>MKELNDLEKKYNAHIGVYALDTKSGKEVKFNSDKRFAYASTSKAINSAILLEQVPYNKLNKKVHINKDDIVAYSPILEKYVGKDITLKALIEASMTYSDNTANNKIIKEIGGIKKVKQRLKELGDKVTNPVRYEIELNYYSPKSKKDTSTPAAFGKTLNKLIANGKLSKE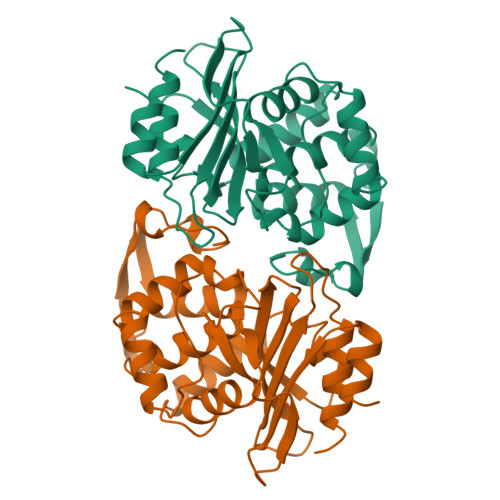NKKFLLDLMLNNKSGDTLIKDGVPKDYKVADKSGQSTYASRNDVAFVYPKGQSEPIVLVIFTNKDNKSDKPNDKLISETAKSVMKEF[2x]3-(3-HYDROXY-7,8-DIHYDRO-6H-CYCLOHEPTA[D]ISOXAZOL-4-YL)-L-ALANINE 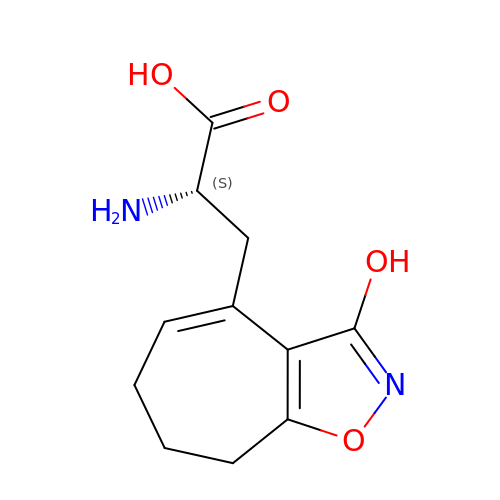| C11 H14 N2 O4 | HJEPOXZLPHUVFE-ZETCQYMHSA-N> MNV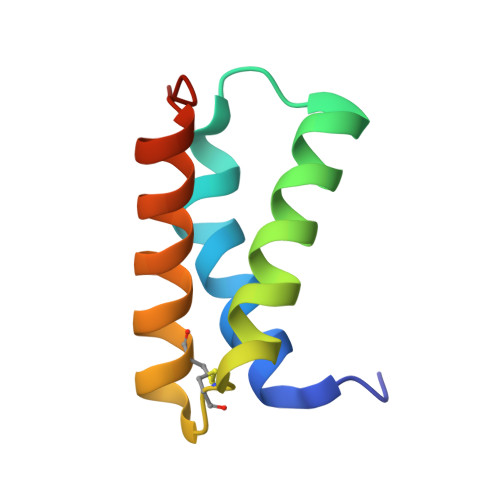DPHFDKFMESGIRHVYMLFENKSVESSEQFYSFMRTTYKNDPCSSDFECIERGAEMAQSYARIMNIKLETE>[3x]MNAIDIAINKLGSVSALAASLGVR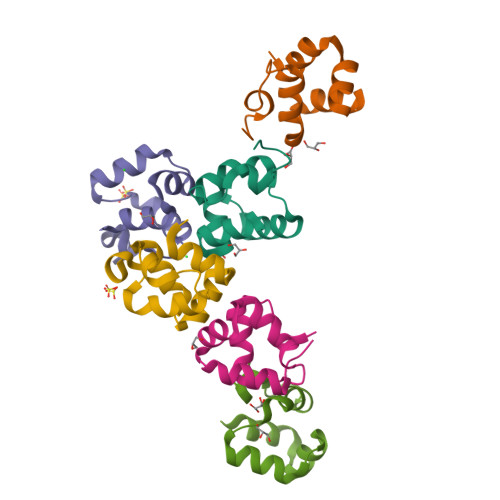QSAISNWRARGRVPAERCIDIERVTNGAVICRELRPDVFGASPAGHRPEASNAAA>[6x]MRGSHHHHHHGSMDKNIIIGAMTALITPFKNGKVDEQSYARLIKRQIENGIDAVVPVGTTGESATLTHEEHRTCIEIAVETCKGTKVKVLAGAGSNATHQAVGLAKFAKEHGADGILSVAPYYNKPTQQGLYEHYKAIAQSVDIPVLLYNVPGRTGCEISTDTIIKLFRDCENIYGVKEASGNIDKCVDLLAHEPRMMLISGEDAINYPILSNGGKGVI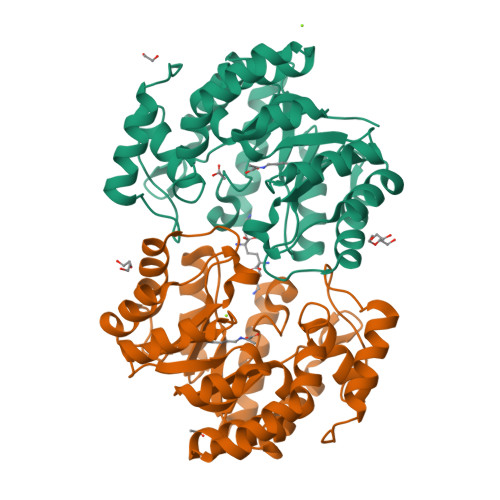SVTSNLLPDMISALTHFALDENYKEAKKINDELYNINKILFCESNPIPIKTAMYLAGLIESLEFRLPLCSPSKENFAKIEEVMKKYKIKGF> GSHMRVTLSSKPQALATPNKEEHGKRKKKGKGLGKKRDPCLRKYKDFCIHGECK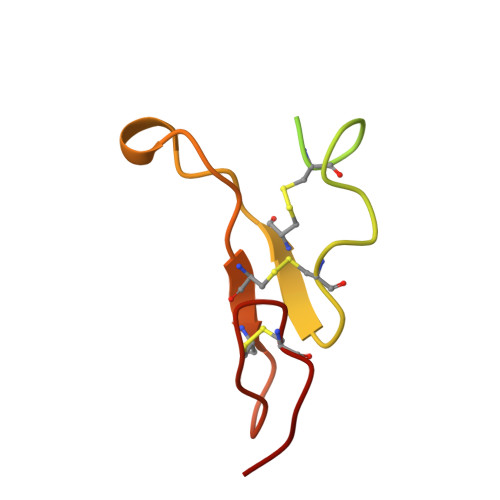YVKELRAPSCICHPGYHGERCHGLS> MFGVKDAIFKIKRSIAGTDSSDSTAYTTASESSPQLKDSHNPFRNKTTSERTIVEEGSLPPVRLNGYLPSTKNKLLTPEMCDEIRTLMPTRIQLY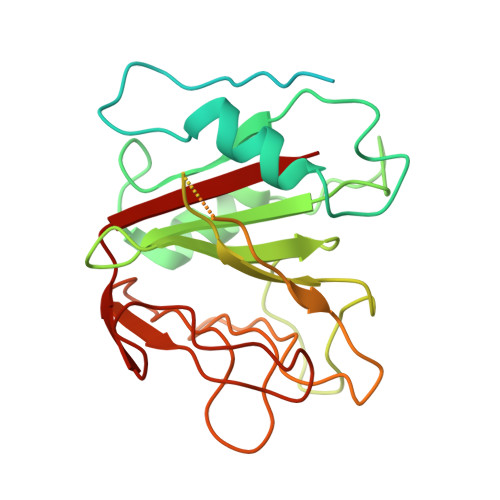TEWNLLYSLEQHGSSLHSLYSNVAPDSKEFRRVGYVLVIKDRKNGIFGAYSNEAFHPNEHRQYTGNGECFLWKLDKVPDVNISEKEESEQEGKEGKEEGDKEERWRFSGYPYTGVNEFAIYCTSEFLSMGAGDGHYGLLCDDGLLHGVSNPCQTYGNEVLSKEGKKFSIVALEVWRVG> MQIGHPSPPPEKKELRKVAHLTGKSNSRSMPLEWEHELGLALLSGVKYKKGGLVINETGLYFVYSKVYFRGQSCNNLPLSHKVYMRNSKYPQDLVMMEGKMMSYCT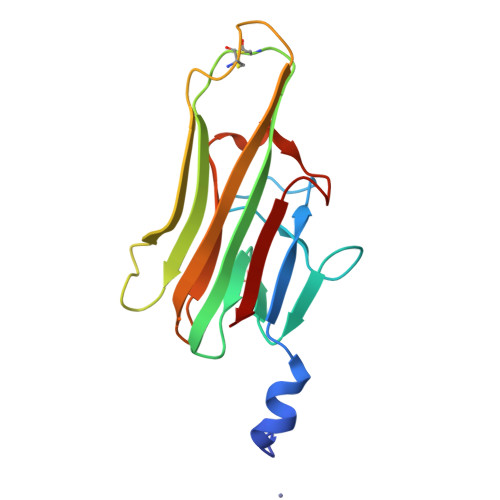TGQMWARSSYLGAVFNLTSADHLYVNVSELSLVNFEESQTFFGLYKL>EVKLILYHWTHSFSSQKVRLVIAEK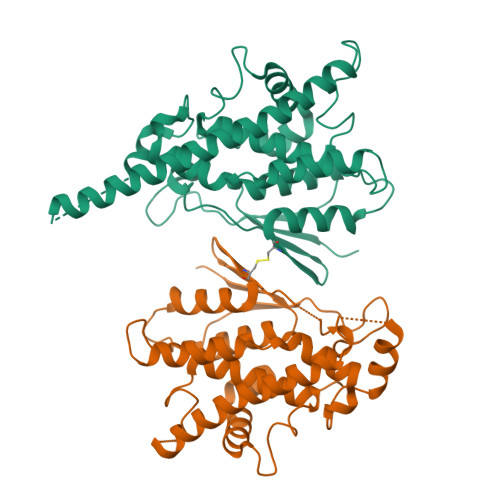ALKCEEHDVSLPLSEHNEPWFMRLNSTGEVPVLIHGENIICEATQIIDYLEQTFLDERTPRLMPDKESMYYPRVQHYRELLDSLPMDAYTHGCILHPELTVDSMIPAYATTRIRSQIGNTESELKKLAEENPDLQEAYIAKQKRLKSKLLDHDNVKYLKKILDELEKVLDQVETELQRRNEETPEEGQQPWLCGESFTLADVSLAVTLHRLKFLGFARRNWGNGKRPNLETYYEHVLKRKTFNKVLGHVNNILIS[2x]>[2x]MSYYHHHHHHLESTSLYKKALAYTLPQLPYAYDALEPHIDARTMEIHHTKHHQTYVDNA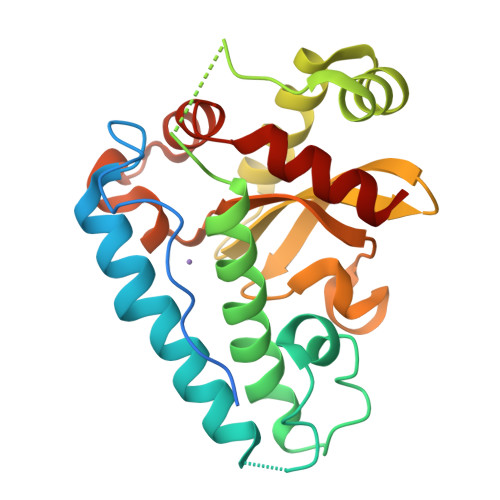NKALEGTEFADLPVEQLIQQLDRVPADKKGALRNNAGGHANHSMFWQIMGQGQGQNGANQPSGELLDAINSAFGSFDAFKQKFEDAAKTRFGSGWAWLVVKDGKLDVVSTANQDNPLMGEAIAGVSGTPILGVDVWEHAYYLNYQNRRPDYLAAFWNVVNWDEVSKRYAAAK>[4x]MHHHHHAIYNVEVETGDREHAGTDATITIRITGAKGRTDYLKLDKGSFEAGSKEQYTVQGFDVGDIQLIELHSDGGGYWSGDPDWFVNRVIIISSTQDRVYSFPCFRWVIKDMVLFPGEATLPFNEVPAIVSEQRQKELEQRKLTYQWDYVSDDMPGNIKAKTHDDLPRDVQFTDEKSRSYQESRKAALVNLGIGSLFTMFENWDSYDDYHILYRNWILGGTPNMADRWHEDRWFGYQFLNGANPVILTRCDALPSNFPVTNEHVNASLDRGKNLDEEIKDGHIYIVDFKVLVGAKSYGGPVLEDIGYKVPDHLKHDEADIRYCAAPLALFYVNKLGHLMPIAIQINQEPGPENPIWTPHEENEHDWMMAK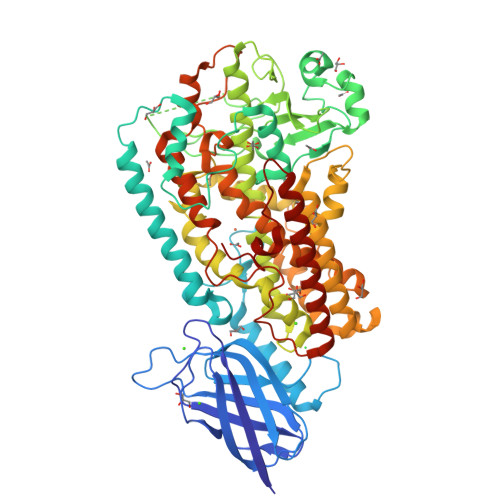FWLGVAESNFHQLNTHLLRTHLTTESFALSTWRNLASAHPIFKLLQPHIYGVLAIDTIGRKELIGSGGIVDQSLSLGGGGHVTFMEKCFKEVNLQDYHLPNALKKRGVDDPSKLPGFYYRDDGLALWEAIETFIGEIIAIFYKNDDDVKRDNEIQSWIYDVHKNGWRVNPGHQDHGVPASFESREQLKEVLTSLVFTFSCQHAAVNFSQKDHYGFTPNAPAILRHPPPKKKGEATLQSILSTLPSKSQAAKAIATVYILTKFSEDERYLGNYSATAWEDKDALDAINRFQDKLEDISKKIKQRNENLEVPYIYLLPERIPNGTAI>MAHHHHHHVGTSFRGKNAVVTGGAGGIGLQVSKQLLAAGAAKVAIIDLQDNLEEFVKLRAAHPTQSV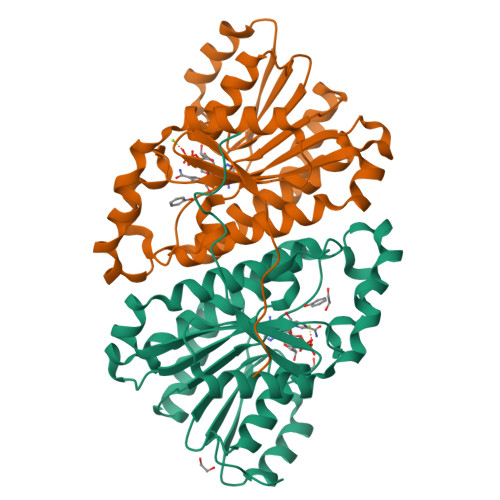MIIKMDVANKKGVEATYEEIAKTFGNIDIVVNVAGIFNDKDVQRTLLVNLGGIINSTLSALPYMGKDNGGKGGIVVNMSSVVGLDPMFIIPVYGATKAGIINFTRCLANEKYYQRSGIKFVTVCPGATMTDMFTNFTEKIIFPETSDETYRILDRLNKQSAADVSRCILNVLEKDKNGAVYVIEGKRVYPLEIKPQWTGKEQAL[2x]> QTIQSIPQKGFFGHPRGLGVLFFVEFWERFSYYGMRAMLIFYMYFAIHQNGLGIDKTTAMSIMSVYGALIYMSSIPGAWIADRITGTRGATLLGAVLIIIGHICLSLPFALFGLFSSMFFIIIGSGLMKPNISNIVGRLYPENDTRIDAGFVIFYMSVNLGALISPIILQHFVDIRNFHGGFLLAAIGMALGLVWYLLFNRKNLGSVGMKPTNPLSKEEKRKYGMIIGIIVAIVIVVLLVTYYTHTLSFDLISNTVLVLGVALPIIYFTTMLRSKDVTDGERSRVKAFIPLFILGMLFWSIQEQGSNVLNIYGLERSDMQLNLFGWTTRFGEALFQSINPLFILLFAPVISMIWLKMGKKQPSLAIKFSIGTLLAGLSYILIGLVGLGYGHTQFSVNWVILSYVICVIGELCLSPTGNSAAVKLAPKAFNAQMMSVWLLTNASAQAINGTLVKLIKPLGQTNYFIFLGTVAIVITLIILVFSPKITKA

Recently we discovered a prokaryotic homolog of PepT1 from the bacterium Staphylococcus hominis, PepTSh, which was able to transport a natural thioalcohol-conjugated peptide, exhibiting structural characteristics similar to prodrug molecules. PepT1 and PepT2 belong to the much larger POT or PTR family of proton-coupled oligopeptide transporters, with homologs found in all domains of life except the archaea. POT family transporters belong to the major facilitator superfamily (MFS) of secondary active transporters, and use the proton electrochemical gradient to drive the concentrative uptake of di- and tripeptides into the cell. To address this question and understand how peptide-based prodrugs and nonproteinogenic drug molecules are recognized and transported via the SLC15 family, we determined the crystal structure of a bacterial POT family member in complex with both valacyclovir and 5-aminolevulinic acid at 3.1-Å and 2.5-Å resolution, respectively.

Following extensive screening, a crystal structure of PepTSh in complex with valacyclovir was subsequently determined using the in meso crystallization method and refined to a final resolution of 3.1 Å. PepTSh adopts an almost identical inward open conformation to that obtained in our previous study, with a root mean square deviation (rmsd) of 0.499 Å for 480 Cα atoms. The valacyclovir drug molecule was clearly observed sitting in the central peptide binding site, coordinating a single water molecule. The valine end of valacyclovir orientates toward the extracellular gate (TMs 1, 2 and 7, 8), which is closed, and the nucleoside part of the drug orientates toward the intracellular gate (TMs 4, 5 and 10, 11), which is open. Valacyclovir makes a number of specific interactions to side chains that are strictly conserved between PepTSh and both PepT1 and PepT2. The amino terminus interacts with a conserved glutamate, E418 (E595, human PepT1 numbering) on TM10 and through a hydrogen bond to an asparagine on TM8, N347 (N329). The carbonyl group makes a hydrogen bond to a conserved asparagine, N167 (N171) on TM5, and the ester bond, which links the l-valine to the acyclovir, interacts with tyrosine Y41 (Y40) on TM1. The acyclovir ether group interacts with another conserved tyrosine, Y79 (Y64) on TM2 and the nucleoside portion of the drug makes a distinctive pi-pi stacking interaction with tyrosine Y163 (Y167), also on TM5. The only nonconserved interaction is made between the nucleoside hydroxyl and N426 on TM10, which in PepT1 is a leucine (L630). Removal of Y163 abrogated valacyclovir recognition, underscoring its importance.>[4x]MSKNIGLNAIEMSYLRQSLSLSAAQVGQLTNHSEAEVLAWENAETQAPELAQKKLLDIDDIIEMQVLNTTDGIEALFKKEPKRHLAFVVYPTQAIYTQYNPEFLSS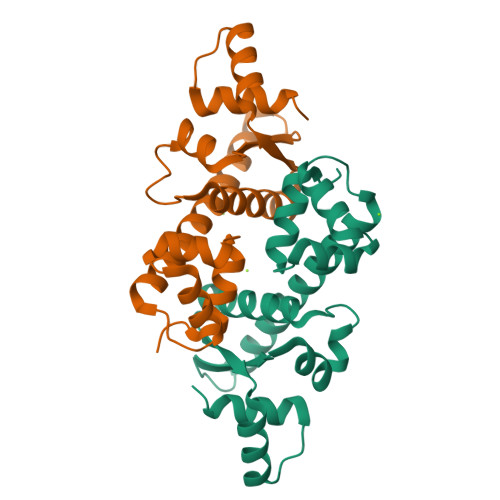LPLTELYNTAAWRIKKECKLVLEVDVSLINLNVEAYKAYREQNGLSESRESRAKWAATQL> MGTEGGAMIRTVALVGHAGSGKTTLTEALLYKTGAKERRGRVEEGTTTTDYTPEAKLHRTTVRTGVAPLLFRGHRVFLLDAPGYGDFVGEIRGALEAADAALVAVSAEAGVQVGTER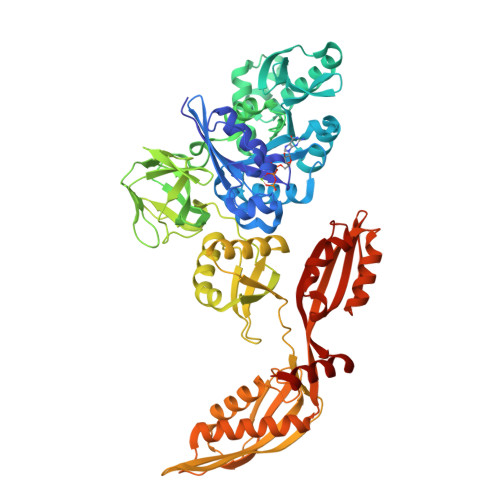AWTVAERLGLPRMVVVTKLDKGGDYYALLEDLRSTLGPILPIDLPLYEGGKWVGLIDVFHGKAYRYENGEEREAEVPPEERERVQRFRQEVLEAIVETDEGLLEKYLEGEEVTGEALEKAFHEAVRRGLLYPVALASGEREIGVLPLLELILEALPSPTERFGDGPPLAKVFKVQVDPFMGQVAYLRLYRGRLKPGDSLQSEAGQVRLPHLYVPMGKDLLEVEEAEAGFVLGVPKAEGLHRGMVLWQGEKPESEEVPFARLPDPNVPVALHPKGRTDEARLGEALRKLLEEDPSLKLERQEETGELLLWGHGELHLATAKERLQDYGVEVEFSVPKVPYRETIKKVAEGQGKYKKQTGGHGQYGDVWLRLEPASEYGFEWRITGGVIPSKYQEAIEEGIKEAAKKGVLAGFPVMGFKAIVYNGSYHEVDSSDLAFQIAASLAFKKVMAEAHPVLLEPIYRLKVLAPQERVGDVLSDLQARRGRILGMEQEGALSVVHAEVPLAEVLEYYKALPGLTGGAGAYTLEFSHYAEVPPHLAQRIVQERAQEG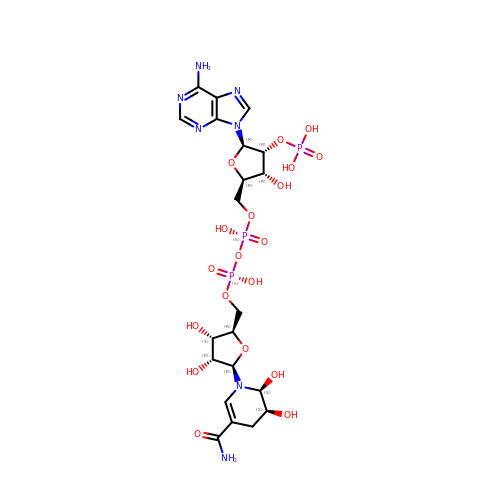5,6-DIHYDROXY-NADP | C21 H32 N7 O19 P3 | LRAVAOPKUBJONV-IVCJQJMGSA-N> AKNECHPERTDGCQHFCLPGQESYTCSCAQGYRLGEDHKQCVPHDQCACGVLTSEKRAPDLQDLPWQVKLTNSEGKDFCGGVIIRENFVLTTAKCSLLHRNITVKTYFNRTSQDPLMIKITHVH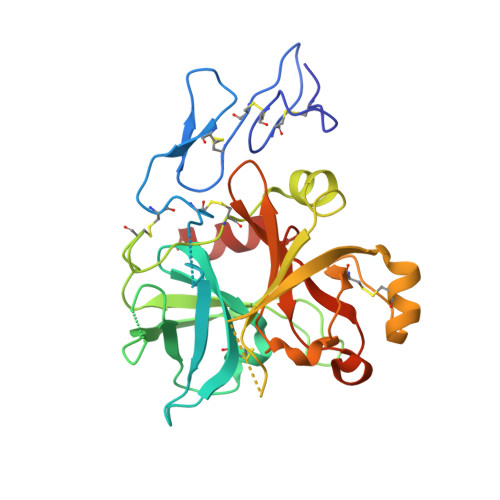VHMRYDADAGENDLSLLELEWPIQCPGAGLPVCTPEKDFAEHLLIPRTRGLLSGWARNGTDLGNSLTTRPVTLVEGEECGQVLNVTVTTRTYCERSSVAAMHWMDGSVVTREHRGSWFLTGVLGSQPVGGQAHMVLVTKVSRYSLWFKQIMNAHHHHHH>[2x]MDSTKEKCDSYKDDLLLRMGLNDNKAGMEGLDKEKINKIIMEATKGSRFYGNELKKEKQVNQRIENMMQQKA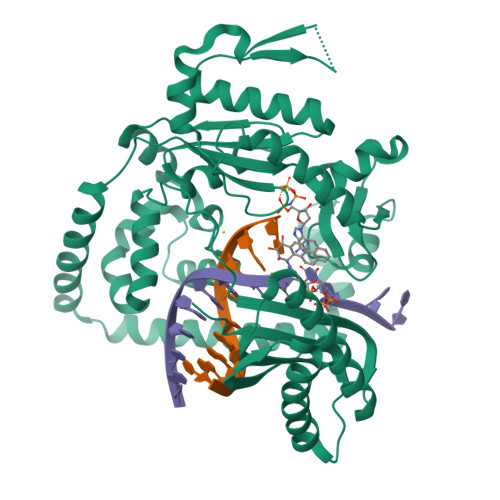QITSQQLRKAQLQVDRFAMELEQSRNLSNTIVHIDMDAFYAAVEMRDNPELKDKPIAVGSMSMLSTSNYHARRFGVRAAMPGFIAKRLCPQLIIVPPNFDKYRAVSKEVKEILADYDPNFMAMSLDEAYLNITKHLEERQNWPEDKRRYFIKMGSSVENDNPGKEVNKLSEHERSISPLLFEESPSDVQPPGDPFQVNFEEQNNPQILQNSVVFGTSAQEVVKEIRFRIEQKTTLTASAGIAPNTMLAKVCSDKNKPNGQYQILPNRQAVMDFIKDLPIRKVSGIGKVTEKMLKALGIITCTELYQQRALLSLLFSETSWHYFLHISLGLGSTHLTRDGERKSMSVERTFSEINKAEEQYSLCQELCSELAQDLQKERLKGRTVTIKLKNVNFEVKTRASTVSSVVSTAEEIFAIAKELLKTEIDADFPHPLRLRLMGVRISSFPNEEDRKHQQR>GPGSMDFRIGQGYDVHQLVPGRPLIIGGVTIPYERGLLGHSDADVLLHAITDALFGAAALGDIGRHFSDTDPRFKGADSRALLRECASRVAQAGFAIRNVDSTIIAQAPKLAPHIDAMRANIAADLDLPLDRVNVKAKTNEKLGYLGRG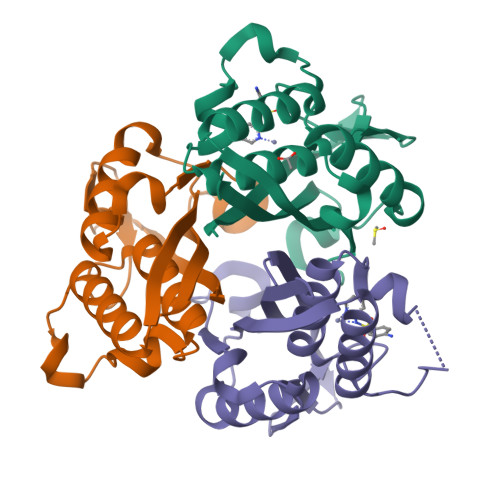EGIEAQAAALVVREAAA[3x]> MGSSHHHHHHSQDPENLYFQGSAANADFELFRVFLEKTCGIVLGSNKQYLVSSRLNKLMEQQGIKSLGELVQRIQTQR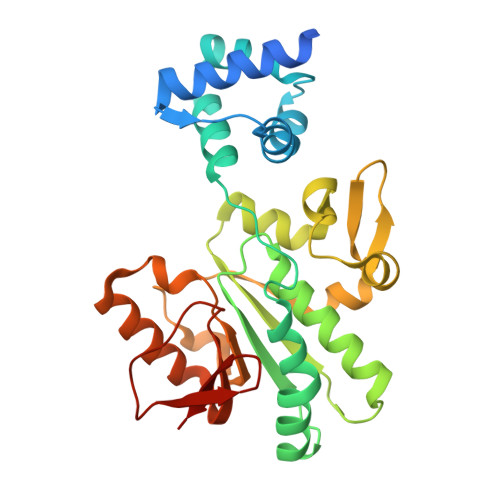GGLREMVVDAMTTNETLWFRDTYPFEVLKQRVLPELIKANGGQRLRIWSAACSSGQEPYSLSMAIDEFEKTNLGQLKAGVQIVATDLSGSMLTAAKAGEYDTLAMGRGLSPERLQRYFDAKGPGRWAVKPAIRSRVEFRALNLLDSYASLGKFDMVFCRNVLIYFSAEVKRDILLRIHGTLKPGGYLFLGASEALNNLPDHYQMVQCSPGIIYRAK> 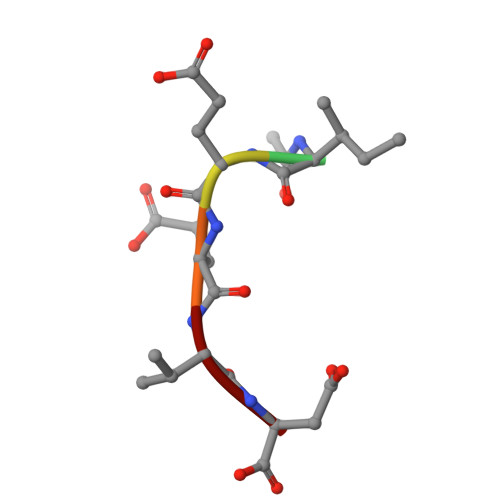XIEEVD(2R)-2-[({1-[3-({(2R,3R,4R,5S,6R)-3-(acetylamino)-4,5-bis(acetyloxy)-6-[(acetyloxy)methyl]tetrahydro-2H-pyran-2-yl}oxy)propyl]-1H-1,2,3-triazol-4-yl}methyl)(biphenyl-4-ylsulfonyl)amino]-3-methylbutanoic 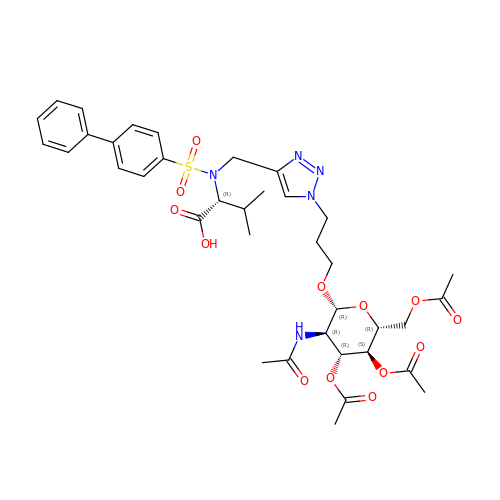acid (non-preferred name) | C37 H47 N5 O13 S | GRIPTHDAFNBNAB-HTJFLOPLSA-N Spermidine/spermine N-acetyltransferases (SSATs) are catabolic enzymes that acetylate polyamines and are critical for maintaining intracellular polyamine homeostasis. SpeG is an SSAT protein found in a variety of bacteria, including the human pathogen Vibrio cholerae. This protein adopts a dodecameric structure and contains an allosteric site, making it unique compared to other SSATs. The allosteric site is located between monomers that form the hexamers of the dodecamer, and some evidence has been provided that shows when polyamine binds to these sites, the dodecamer tightens.

The first construct (R3C1) removes the residues that form a portion of β7 and a portion of the beta-turn of the β6-β7 region of the protein and replaces them with the corresponding residues from hSSAT1 in its linear sequence. Since the N152 residue of VcSpeG is replaced with a positively charged lysine from hSSAT1 and it normally forms an H-bond with R25 of Region 1, it is possible this substitution would repel the interaction between these two regions. Despite crystallizing in a range of crystallography space groups, six structures adopted the apo-conformation of VcSpeG. The replacement of the beta-turn (four amino acids; FFIN (F149-N152)) of Region 3 of the VcSpeG protein (R3C1) caused the activity to decrease 26-fold compared to WT. The R3C1 model showed the secondary structures of this region generally adopted the same conformation as WT. When we examined the residues of this construct compared to the WT protein more closely, the homology models showed substitutions of F149 to arginine and F150 to leucine affect their interactions with Region 1. For example, the models showed R149 formed an H-bond with the adjacent E148 residue, which disrupted the π-π interactions originally held by F32 and F149. Additionally, when F150 was replaced by leucine in the model, the T-shaped π-π interaction originally formed between F150 and Y155 in the WT structure was disrupted. Substitution of N152 to lysine also removed the H-bond typically seen between R25 and N152 in the WT structure. However, when we examined the chimera with a four-residue substitution (R3C1), including both of the F149 and N152 residues exchanged with positively charged residues, we saw a much more substantial decrease in activity.

>[3x]MNSQLTLRALERGDLRFIHNLNNNRNIMSYWFEEPYESFDELEELYNKHIHDNAERRFVVEDAQKNLIGLVELIEINYIHRSAEFQIIIAPEHQGKGFARTLINRALDYSFTILNLHKIYLHVAVENPKAVHLYEECGFVEEGHLVEERLFKGRYQDVKRMYILQSKYLNRSE> XXXXXXXTGLSEMRLEKDRFSVNLDVKHFSPEELKVKVLGDVIEVHGKHEERQDEHGFISREFHRKYRIPADVDPLTITSSLSSDGVLTVNGPRKQVSGPERTIPITR;> SVNLDVKHFSPEELKVKVLGDVIEVHGKHEERQDEHGFISREFHRKYRIPADVDPLTITSSLS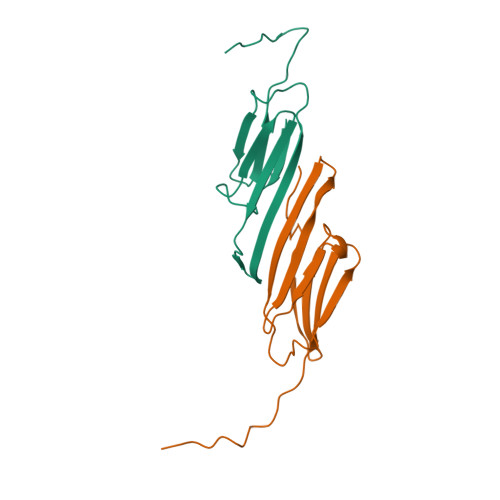SDGVLTVNGPRKQVSGPERTIPITR> GPMALQMVTVGHNIALIQPGFSLMNFDGQVFFFGQKGWPKRSCPTGVFHFDIKQNHLKLKPAIFSKDSCYLPPLRYPATCSYKGSIDSDKHQYIIHGGKTPNNELSDKIYIMSVACKNNKKVTFRCTEKDLVGDVPEPRYGHSIDVVYSRGKSMGVLFGGRSYMPSTQRTTEKWNSVADCLPHVFLIDFEFGCATSYILPELQDGLSFHVSIARNDTVYILGGHSLASNIRPANLYRIRVDLPLGTPAVNCTVLPGGISVSSAILTQTNNDEFVIVGGYQLENQKRMVCSLVSLGDNTIEISEMETPDWTSDIKHSKIWFGSNMGNGTI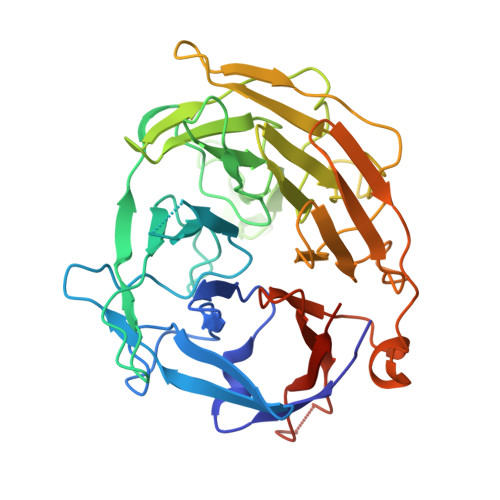FLGIPGDNKQAMSEAFYFYTLRCSEEDLSEDQKI>MNDYSRQNFLDLNLFRGLGEDPAYHPPVLTDRPRDWPLDRWAEAPRDLGYSDFSPYQWRGLRMLKDPDTQAVYHDMLWELRPRTIVELGVYNGGSLAWFRDLTKIMGIDCQVIGIDRDLSRCQIPASDMENITLHQGDCSDLTTFEHLREMAHPLIFIDDAHANTFNIMKWAVDHLLEEGDYFIIE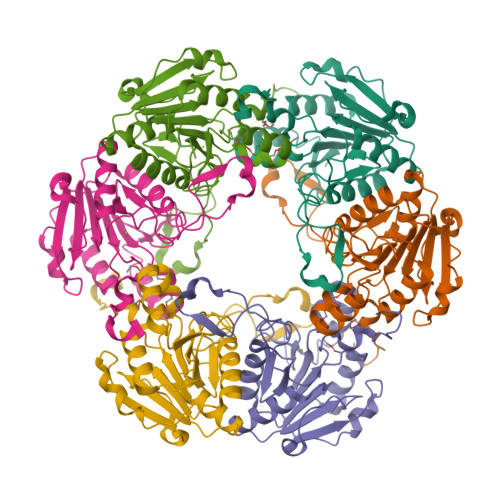DMIPYWYRYAPQLFSEYLGAFRDVLSMDMLYANASSQLDRGVLRRVAAKQ[6x]>VQSDTHIFIIMGASGDLAKKKIYPTIWWLFRDGLLPENTFIVGYARSRLTVADIRKQSEPFFKATPEEKLKLEDFFARNSYVAGQYDDAASYQRLNSHMNALHLGSQANRLFYLALPPTVYEAVTKNIHESCMSQIGWNRIIVEKPFGRDLQSSDRLSNHISSLFREDQIYRIDHYLGKEMVQNLMVLRFANRIFGPIWNRDNIACVILTFKEPFGTEGRGGYFDEFGIIRDVMQNHLLQMLCLVAMEKPASTNSDDVRDEKVKVLKCISEVQANNVVLGQYVGNPDGEGEATKGYLDDPTVPRGSTTATFAAVVLYVENERWDGVPFILRCGKALNERKAEVRLQFHDVAGDIFHQQCKRNELVIRVQPNEAVYTKMMTKKPGMFFNPEESELDLTYGNRYKNVKLPDAYERLILDVFCGSQMHFVRSDELREAWRIFTPLLHQIELEKPKPIPYIYGSRGPTEADELMKRVGFQYEGTYKWVNPH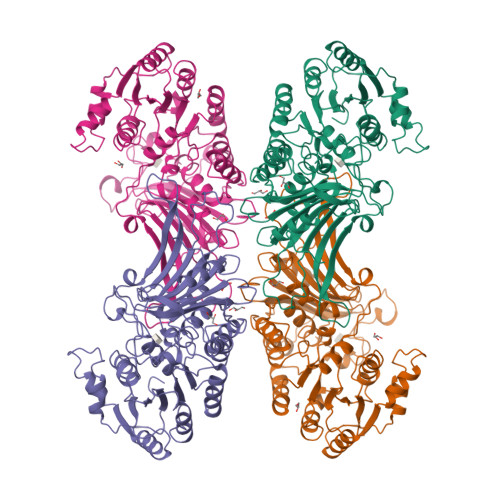KL[2x]> TAYYAQALQSVPETQVSQLDNGVRVASEQSSQPTCTVGVWIDAGSRYESEKNNGAGYFLEHLAFKGTKNRPQNALEKEVESMGAHLNAYSSREHTAYYIKALSKDVPKAVELLADIVQNCSLEDSQIEKERDVIVRELQENDTSMREVVFNYLHATAFQGTGLAQSVEGPSENIRKLSRADLTEYLSTHYTAP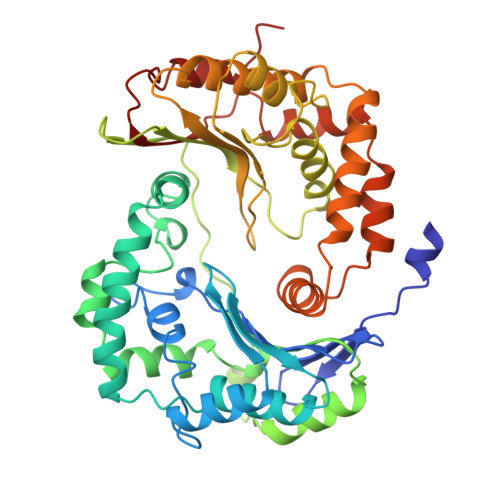RMVLAAAGGVEHQQLLELAQKHFGGVPFTYDDDAVPTLSKCRFTGSQIRHREDGLPLAHVAIAVEGPGWAHPDLVALQVANAIIGHYDRTYGGGLHSSSPLASIAVTNKLCQSFQTFSICYSETGLFGFYFVCDRMSIDDMMFVLQGQWMRLCTSISESEVLRGKNFLRNALVSHLDGTTPVCEDIGRELLTYGRRIPLEEWEERLAEVDARMVREVCSKYIYDQCPAVAGPGPIEQLPDYNRIRSGMFWLRF> GAKDQLETLKRIIEKSEGISILINGEDLSYPREVSLELPEYVEKFPPKASDVLEIDPEGENIGIDDIRTIKDFLNYSPELYTRKYVIVHDCERMTQQAANAFLKALEEPPEYAVIVLNTRRW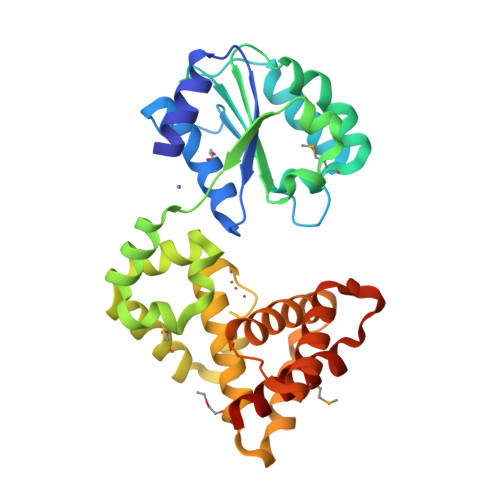HYLLPTIKSRVFRVVVNVPKEFRDLVKEKIGDLWEELPLLERDFKTALEAYKLGAEKLSGLMESLKVLETEKLLKKVLSKGLEGYLACRELLERFSKVESKEFFALFDQVTNTITGKDAFLLIQRLTRIILHENTWESVEDQKSVSFLDSILRVKIANLNNKLTLMNILAIHRERKRGVNAWS N-[1-(N'-CYANO-N-[3-(DIFLUOROMETHOXY)PHENYL]CARBAMIMIDOYL)-3-(3,4-DICHLOROPHENYL)-4,5-DIHYDRO-1H-PYRAZOL-4-YL]-N-ETHYL-2-HYDROXYACETAMIDE | C22 H20 Cl2 F2 N6 O3 | 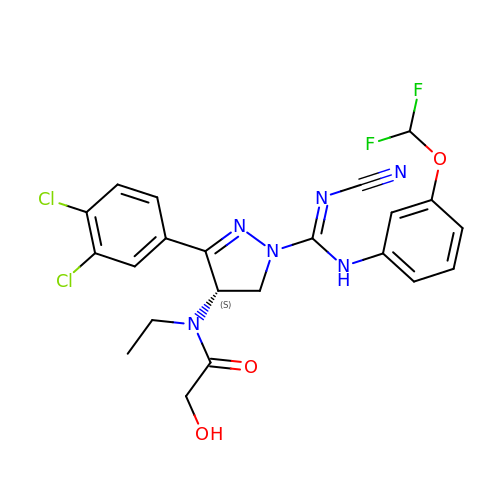OTTJIRVZJJGFTK-SFHVURJKSA-N>[4x]GPLGSDYIIKEKTVLLQKKDSEGFGFVLRGAKAQTPIEEFTPTPAFPALQYLESVDEGGVAWRAG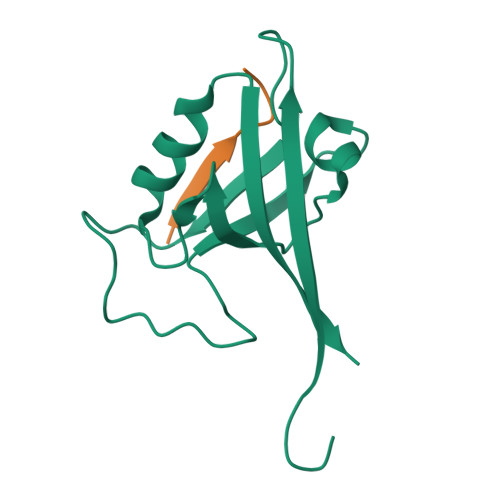LRMGDFLIEVNGQNVVKVGHRQVVNMIRQGGNTLMVKVVMVTRHPDM;>[4x]EESTSFQGP> PVTINNFNYNDPIDNNNIIMMEPPFARGTGRYYKAFKITDRIWIIPERYTFGYKPEDFNKSSGIFNRDVCEYYDPDYLNTNDKKNIFLQTMIKLFNRIKSKPLGEKLLEMIINGIPYLGDRRVPLEEFNTNIASVTVNKLISNPGEVERKKGIFANLIIFGPGPVLNENETIDIGIQNHFASREGFGGIMQMKFCPEYVSVFNNVQENKGASIFNRRGYFSDPALILMHELIHVLHGLYGIKVDDLPIVPNEKKFFMQSTDAIQAEELYTFGGQDPSIITPSTDKSIYDKVLQNFRGIVDRLNKVLVCISDPNININIYKNKFKDKYKFVEDSEGKYSIDVESFDKLYKSLMFGFTETNIAENYKIKTRASYFSDSLPPVKIKNLLDNEIYTIEEGFNISDKDMEKEYRGQNKAINKQAYEEISKEHLAVYKIQMCKSVKAPGICIDVDNEDLFFIADKNSFSDDLSKNERIEYNTQSNYIENDFPINELILDTDLISKIELPSENTESLTDFNVD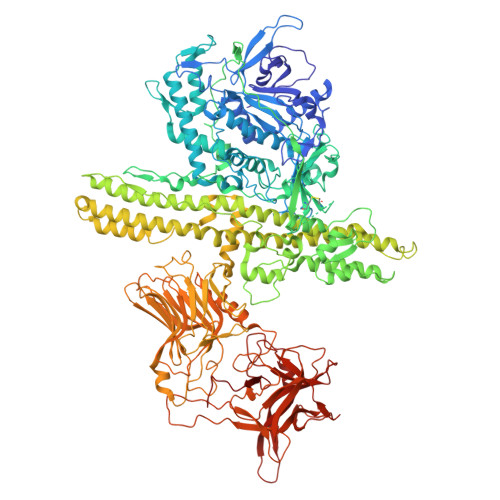VPVYEKQPAIKKIFTDENTIFQYLYSQTFPLDIRDISLTSSFDDALLFSNKVYSFFSMDYIKTANKVVEAGLFAGWVKQIVNDFVIEANKSNTMDKIADISLIVPYIGLALNVGNETAKGNFENAFEIAGASILLEFIPELLIPVVGAFLLESYIDNKNKIIKTIDNALTKRNEKWSDMYGLIVAQWLSTVNTQFYTIKEGMYKALNYQAQALEEIIKYRYNIYSEKEKSNINIDFNDINSKLNEGINQAIDNINNFINGCSVSYLMKKMIPLAVEKLLDFDNTLKKNLLNYIDENKLYLIGSAEYEKSKVNKYLKTIMPFDLSIYTNDTILIEMFNKYNSEILNNIILNLRYKDNNLIDLSGYGAKVEVYDGVELNDKNQFKLTSSANSKIRVTQNQNIIFNSVFLDFSVSFWIRIPKYKNDGIQNYIHNEYTIINCMKNNSGWKISIRGNRIIWTLIDINGKTKSVFFEYNIREDISEYINRWFFVTITNNLNNAKIYINGKLESNTDIKDIREVIANGEIIFKLDGDIDRTQFIWMKYFSIFNTELSQSNIEERYKIQSYSEYLKDFWGNPLMYNKEYYMFNAGNKNSYIKLKKDSPVGEILTRSKYNQNSKYINYRDLYIGEKFIIRRKSNSQSINDDIVRKEDYIYLDFFNLNQEWRVYTYKYFKKEEEKLFLAPISDSDEFYNTIQIKEYDEQPTYSCQLLFKKDEESTDEIGLIGIHRFYESGIVFEEYKDYFCISKWYLKEVKRKPYNLKLGCNWQFIPKDEGWTE> GSMSVQAEIGILDHVDGSSEFVSQDTKVICSVTGPIEPKARQELPTQLALEIIVRPAKGVATTREKVLEDKLRAVLTPLITRHCYPRQLCQI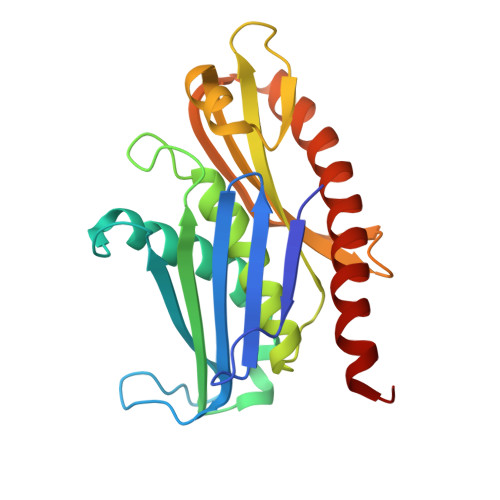TCQILESGEDEAEFSLRELSCCINAAFLALVDAGIALNSMCASIPIAIIKDTSDIIVDPTAEQLKISLSVHTLALEFVNGGKVVKNVLLLDSNGDFNEDQLFSLLELGEQKCQELVTNIRRIIQDNISPRLVV>SELAARCLIILFQQLVELARLAIESGDEELLRRVSEWLEEVIKDMRRVVEQALREGNSELAARILIILFQQLVELARLAIESGDEELLRRVSEWLEEVIKDMRRVVEQALREGNSELAARILIILFQQLVELARLAIESGDEELLRRVSEWLEEVIKDMRRVVEQALREGNSELAARILIILFQQLVELARLAIESGDEELLRRVSEWLEEVIKDMRRVVEQALREGNSELAARILIILFQQLVELARLAIESGDEELLRRVSEWLEEVIKDMRRVVEQALREGNSELAARILIILFQQLVELARLAIESGDEELLRRVSEWLEEVIKDMRRVVEQALREGNSELAARILIILFQQLVELARLAIESGDEELLRRVSEWLEEVIKDMRRVVEQALREGNSELACRILII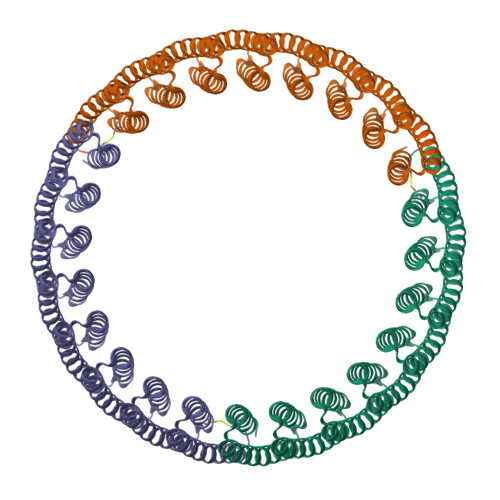LFQQLVELARLAIESGDEELLRRVSEWLEEVIKDMRRVVEQALREGN[3x]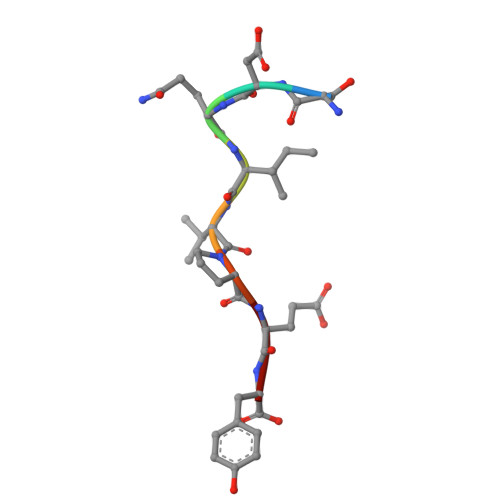> SDQIVPEY The nucleocapsid is surrounded by a bilayer lipid membrane and on the outside of the membrane are the 180 pairs of envelope (E) and membrane (M) proteins. The E and M proteins are arranged with icosahedral symmetry with each asymmetric unit containing three pairs of E and M heterodimers. The E protein ectodomain consists of three domains: DI, DII and DIII121314. E protein plays an important role in virus entry into host cell as it binds to receptors and facilitates fusion of the virus to the endosomal membrane.

As the DENV3-Fab 5J7 complex was formed at 37 °C, we also determined a 7-Å resolution cryo-EM structure of the uncomplexed mature DENV3 that had been exposed to 37 °C for 30 min and incubated at 4 °C for 2 h before freezing. Superposition of cryo-EM structures of uncomplexed DENV3 at 28 °C and 37 °C showed similar structures. Therefore, unlike the DENV2 New Guinea C strain3233, the E protein layer of the uncomplexed DENV3 863DK strain does not undergo irreversible conformational changes when exposed to 37 °C. Our uncomplexed DENV3 structure represents the structure that was incubated at 37 °C for 30 mins and then 4 °C for 2 h before freezing. It did not show any structural difference compared with the sample that was grown at 28 °C. This finding suggests that the E proteins on DENV3 do not undergo temperature-irreversible conformational change, as observed in DENV2. However, it is still possible that the E proteins have small conformational changes when kept at 37 °C, thus lowering the binding of HMAb 5J7 to virus before it attaches to cells.

>MRCVGVGNRDFVEGLSGATWVDVVLEHGGCVTTMAKNKPTLDIELQKTEATQLATLRKLCIEGKITNITTDSRCPTQGEAVLPEEQDQNYVCKHTYVDRGWGNGCGLFGKGSLVTCAKFQCLEPIEGKVVQYENLKYTVIITVHTGDQHQVGNETQGVTAEITPQASTTEAILPEYGTLGLECSPRTGLDFNEMILLTMKNKAWMVHRQWFFDLPLPWASGATTETPTWNRKELLVTFKNAHAKKQEVVVLGSQEGAMHTALTGATEIQNSGGTSIFAGHLKCRLKMDKLELKGMSYAMCTNTFVLKKEVSETQHGTILIKVEYKGEDAPCKIPFSTEDGQGKAHNGRLITANPVVTKKEEPVNIEAEPPFGESNIVIGIGDNALKINWYKKGSSIGKMFEATARGARRMAILGDTAWDFGSVGGVLNSLGKMVHQIFGSAYTALFSGVSWVMKIGIGVLLTWIGLNSKNTSMSFSCIAIGIITLYLGAVVQA[3x];>[3x]SVALAPHVGMGLDTRTQTWMSAEGAWRQVEKVETWALRHPGFTILALFLAHYIGTSLTQKVVIFILLMLVTPSMT>MDHHHHHHHHASENLYFQGHMNLDLAYRSFVLGVAGHPQVERLIKHRAKGLVRRYVAGETLEEALKAAEALEREGVHAILDLLGEMVRTEEEARAFQRGLLELVW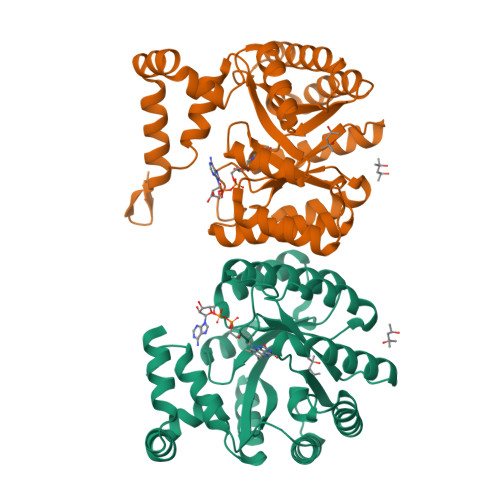ALAGKPWPKYISLKLTQLGLDLSEDLALALLREVLREAEPRGVFVRLDMEDSPRVEATLRLYRALREEGFSQVGIVLQSYLYRTEKDLLDLLPYRPNLRLVKGAYREPKEVAFPDKRLIDAEYLHLGKLALKEGLYVAFATHDPRIIAELKRYTEAMGIPRSRFEFQFLYGVRPEEQRRLAREGYTVRAYVPYGRDWYPYLTRRIAERPENLLLVLRSLVSG[2x]[[(2R,3S,4R,5R)-5-(6-aminopurin-9-yl)-4-oxidanyl-3-phosphonooxy-oxolan-2-yl]methoxy-oxidanyl-phosphoryl] 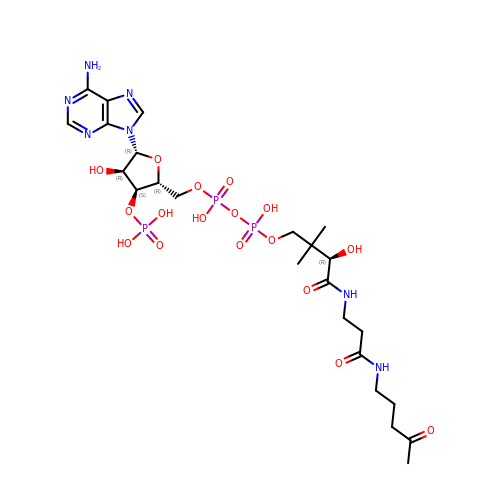[(3R)-2,2-dimethyl-3-oxidanyl-4-oxidanylidene-4-[[3-oxidanylidene-3-(4-oxidanylidenepentylamino)propyl]amino]butyl] hydrogen phosphate | C24 H40 N7 O17 P3 | ZYXBXYCDXPIBJY-NDZSKPAWSA-N D-xylonic acid | C5 H10 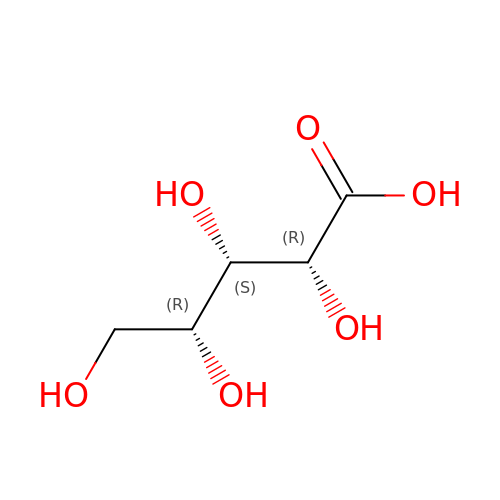O6 | QXKAIJAYHKCRRA-FLRLBIABSA-N> GPLGSMTTPSHLSDRYELGEILGFGGMSEVHLARDLRLHRDVAVKVLRADLARDPSFYLRFRREAQNAAALNHPAIVAVYDTGEAETPAGPLPYIVMEYVDGVTLRDIVH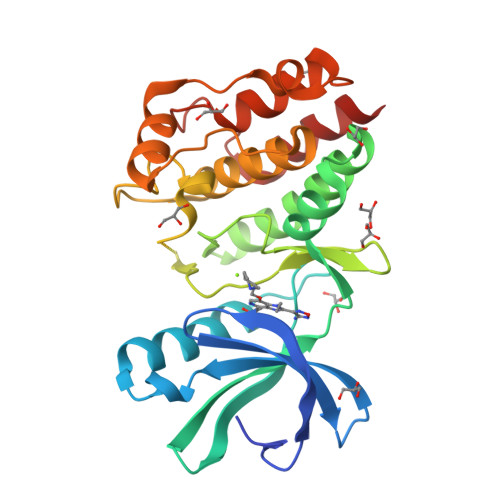TEGPMTPKRAIEVIADACQALNFSHQNGIIHRDVKPANIMISATNAVKVMDFGIARAIADSGNSVTQTAAVIGTAQYLSPEQARGDSVDARSDVYSLGCVLYEVLTGEPPFTGDSPVSVAYQHVREDPIPPSARHEGLSADLDAVVLKALAKNPENRYQTAAEMRADLVRVHNGE>MIQTERAVQQVLEWGRSLTGFADEHAVEAVRGGQYILQRIHPSLRGTSARTGRDPQDETLIVTFYRELALLFWLDDCNDLGLISPEQLAAVEQALGQGVPCALPGFEGCAVLRASLATLAYDRRDYAQLLDDTRCYSAALRAGHAQAVAAERWSYAEYLHNGIDSIAYANVFCCLSLLWGLDMATLRARPAFRQVLRLISAIGRLQNDLHGCDKDRSAGEADNAVILLLQRYPAMPVVEFLNDELAGHTRMLHRVMAEERFPAPWGPLIEAMAAIRVQYYRTSTSRYRSDAVRGG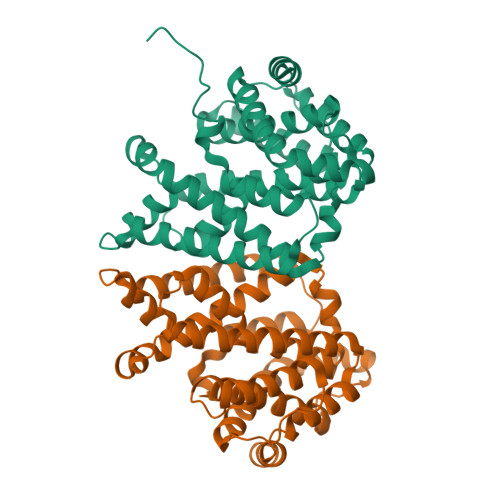QRAPA[4x]hexyl(trihydroxy)borate(1-) | C6 H16 B O3 | 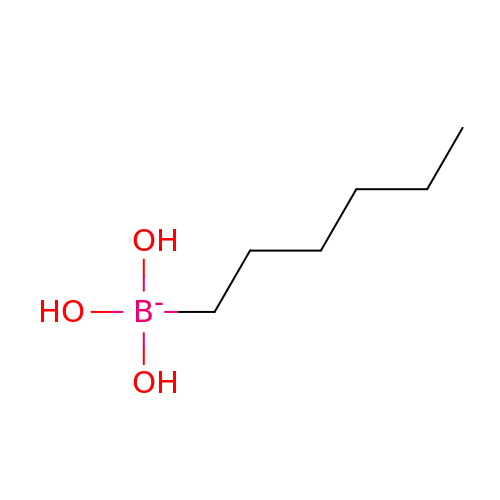ZVNFLSCBVLLZCO-UHFFFAOYSA-N>[2x]GAMEEAVVATEPLTREDLIAYLASGCKSKEKWRIGTEHEKFGFEVNTLRPMKYDQIAELLNSIAERFEWEKVMEGDKIIGLKQGKQSIS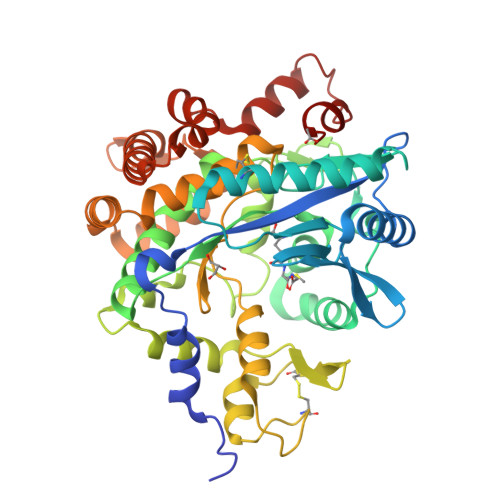LEPGGQFELSGAPLETLHQTCAEVNSHLYQVKAVAEEMGIGFLGMGFQPKWRREDIPTMPKGRYDIMRNYMPKVGSLGLDMMLRTCTVQVNLDFSSEADMIRKFRAGLALQPIATALFANSPFTEGKPNGFLSMRSHIWTDTDKDRTGMLPFVFDDSFGFEQYVDYALDVPMYFAYRNGKYVDCTGMTFRQFLAGKLPCLPGELPTYNDWENHLTTIFPEVRLKRYMEMRGADGGPWRRLCALPAFWVGLLYDEDVLQSVLDLTADWTPAEREMLRNKVPVTGLKTPFRDGLLKHVAEDVLKLAKDGLERRGYKEVGFLNAVTEVVRTGVTPAENLLEMYNGEWGQSVDPVFQELLY> RVTTVGDLAVLEGRSVMIPCHYGPQYASYVKYWCRGSVKDLCTSLVRSDAPRGPAAAGEDKVVMFDDPVQQVFTVTMTELQKEDSGWYWCGVEVGGVWSADVTASLHINVIQGLSVVNSMVSGEEGTSVTVQCLYSQGYRQHEKRWCRSGDWSSCLVTDGEGRYEDQAVEIRDDLTKAFTVTLKGLARRDTGWYWCAAGQQQVAVYILVTPPSH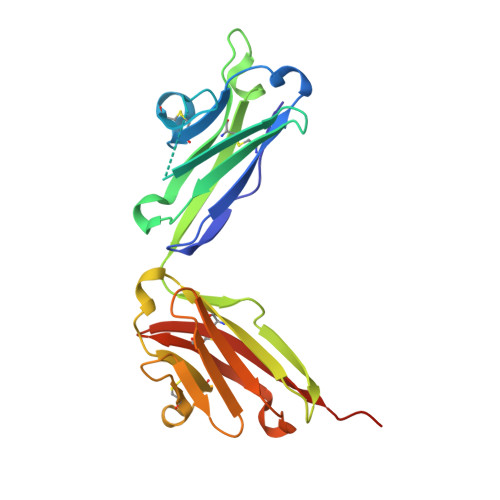HHHHH Here we report the high-resolution structure of an aviadenovirus, the poultry pathogen fowl adenovirus serotype 4 (FAdV-C4). Adenoviruses stand out among the icosahedral, non-enveloped viruses because of their large capsid size (950 Å, ~ 150 MDa), triangulation number (pseudo-T = 25) and complex composition. The capsid facets are formed by 240 trimeric hexons, with twelve pentameric pentons at the vertices. Minor coat proteins IIIa, VI and VIII on the inner capsid surface contribute to modulate the quasi-equivalent icosahedral interactions, along with the genus specific outer proteins IX (in mastadenoviruses) or LH3 (in atadenoviruses).

We obtained high resolution 3D maps for two different FAdV-C4 strains: KR5, and AG234. Model building was carried out for the KR5 map, given that the AG234 map presented a disrupted particle lacking pentons. The structure shows the general characteristics common to all previously solved adenovirus structures: hexons (major capsid protein) and penton base (vertex protein) arranged in a pseudo T = 25 icosahedral particle, with inner cementing proteins IIIa and VIII on the inner capsid surface. In agreement with the LC-MS/MS data, no densities that could be interpreted as genus specific minor coat proteins were present in the map. In addition to these expected results, we found that the FAdV-C4 hexon presents a unique insertion of fourteen amino acids located at the equator of the hexon trimer. The variable loop (VL, diff 3) is quite long in FAdV-C4 (17 vs 6 aa in HAdV-C5) and folds back towards the main body of the monomer, augmenting intramolecular interactions, in sharp contrast to the protruding orientation of the VL in HAdV-C5. The α2 helix in the body domain of HAdV-C5 protein VIII is 22 amino acid long, while its counterpart in FAdV-C4 is shorter (13 residues) and followed by a bend of 115º and another 12-residue α-helix (α2’). Additionally, while in the human and lizard viruses the first helix of the VIII-binding domain is roughly perpendicular to the connecting helix, in FAdV-C4 this helix adopts an oblique orientation, which results in a completely different conformation of the protein in each one of the genera. Interestingly, the N-terminal region of one monomer in hexon 1 (chain B) interlaces with the divergent neck region of VIII, while the N-terminus of one monomer in hexon 2 (chain F) crosses over the head domain of protein VIII, further securing it in a clasp near the AVP cleavage site (ovals, and 7c). Thus, the long N-terminal tail unique to the aviadenovirus hexon in combination with the different fold of protein VIII could play a stabilizing role in the capsid.

>[12x]MAALTPDLTTATPRLQYFHIAGPGTREYLSEDLQQFISATGSYFDLKNKFRQTVVAPTRNVTTEKAQRLQIRFYPIQTDDTSTGYRVRYNINVGDGWVLDMGSTYFDIKGILDRGPSFKPYCGTAYNPLAPKESMFNNWSETAPGQNVSASGQLSNVYTNTSTTKDTTAAQVTKISGVFPNPNQGPGINPLRQVENANTGVLGRFAKSQYNYAYGAYVKPVAADGSQSLTQTPYWIMNNAGTEYLGAVAVEDYTNSLSYPDTMIVPPPEDYDDYNIGTTRALRPNYIGFRDNFINLLYHDSGVCSGTLNSERSGMNVVVELPDRNTELSYQYMLADMMSRHHYFALWNQAVDQYDPEVRVFSNDGYEEGAPSYAFNPEAVGAGEGYGPDLSQIKLYTNNTAANDKNTAVTNATTNFYFGTVPSYEIDISATQRRNFIMANIAEYLPDRYKFSISGFDATSVAPTTYEYMNKRVPLTNVVDMFTNVGARWSIDQMDNVNPFNHHRNWGLKYRSQLLGNSRYVNFHIQVPQKFFAIKNLLLLSGSYTYEWVLRKDPNMILQSSLGNDLRADGASIIYNEVNLMANFMPMDHNTSNQLELMLRNATNDQTFVDYLGAKNALYSVPAGSTALTINIPARTWEGMRGWSFTRIKAAETPQLGAQYDVNFKYSGSIAYSDGGFYLSHTFRNMSILFDTSINWPGNDRLLTPNMFEIKRSVALDTEGFTMSQCDITKDWYLIQMATNYNFVYNGYRFWPDRQYFHYDFLRNFDPMTRQGPNFALPGLFDLVSYTPTTDNSGEQPSQEAVRNNSGFIAPRSWPVWSAHQGESWPANWPYPLCGQQAIQPGQVLSYKKFLCDNYLWTIPFSSDFMYMGELTDLGQNPMYTNNSHSMVINFELDPMDDPTYVYMLYGVFDTVRVNQPERNVLAMAYFRTPFATGNAV;> MWGLQPPTSIPPPPPPTELTPSTYPAMVNGYPPPAASAQSCSSSGGQSELYMPLQRVMAPTGGRNSIKYRDYTPCRNTTKLFYVDNKASDIDTYNKDANHSNFRTTVIHNQDLDADTAATESIQLDNRSCWGGDLKTAVRTNCPNVSSFFQSNSVRVRMMWKRDPPTSTAPPSAVGSGYSVPGAQYKWYDLTVPEGNYALCELIDLLNEGIVQLYLSEGRQNNVQKSDIGVKFDTRNFGLLRDPVTGLVTPGTYVYKGYHPDIVLLPGCAIDFTYSRLSLLLGIGKREPYSKGFVITYEDLQGGDIPALLDLDSVDVNDADGEVIELDNAAPLLHDSAGVSYNVIYDQVTGKPVTAYRSWMLAYNVPNSQANQTTLLTVPDMAGGIGAMYTSLPDTFIAPTGFKEDNTTNLCPVVGMNLFPTYNKIYYQAASTYVQRLENSCQSATAAFNRFPENEILKQAPPMNVSSVCDNQPAVVQQGVLPVKSSLPGLQRVLITDDQRRPIPYVYKSIATVQPTVLSSATLQ;> MSSTEVFGALAPVGRTEVADALSSHANSKDARSLRYEPYANRLIKLQTAMVPPKVDGTSERVAEVVKGLAEQGAIYPDQMGAIHSDLLNRVYTWNSMGVQESIQALVNDVIHGQNKVLQDELARTREIANASMLTRFFDSLYKTVDRGQRNFEGFKKLLRLFVNNVPNAEVYSSGGSFSLQINMGGQSQNINLTNAFDNLKDIWGARWDAVNNPRIGALLTPNTRALLFFVSTFYDYGSMEPGSYLDNLMRLYKEAIRADTDAEGDAIMELGDAGANLNLKFNQYKDTLNYLLQNKPSVPQTGPLEMSPEQESLFKYLMRQLRRALKDGVNSDIAISTMAQYVDPRLYTSNKVFIDKLQNYLLMASARNPYYYKTIVLDPHWVPPAGLYTDNFVIPEMMPNFSDFASELEYGGPSRDEYFDDSPFRPPPQKKFTEKEQADYDSLINFFDSTLGVQSEAGWIADHRLPQAFDGALNVSERTPYNTPLPDDAPMRSRNASVSSATDALGQLKLSGTGGAGFFDSLKPSVGTRRSTGLAKGLAGTGQPPCPWPASVGYASAGYGPARGIRGSGLARRALAARGLRQGKRLRFY;>[2x]MNLLNAAPTPYVWKYNPVTGKCAGAQQNYGATIDWVLPGGNSFAYAADEIRRRFPEPAVTRAITARFEAESDQQPYAGPHETNIITADVVRSGPPPSAVYPFDPSGVQRVQLSGGMMGGRTEGRMQLSGGLTEGRMQLAGGAAGKLPTRARPTLRPPRWCGTTLTGNGLPADYPEMTPDAFKYYLRVQGPSQEVDEPGVMSQRQFMTTFLPAMVPHPFDSESPDAFPAYFSSVYKGTNAFEPVFWQG>EEVKAIRIPVVRLKFGEVAEATSVVVLPVCKAEEGEKKILEAPMEIIAGGDFKVVEAEKGWKRWVVLPSWNPVAAIGKGGVAVSFRDDRKVLPWDGKEEPLLVVADRVRNVVEADDGYYLVVAENGLKLEKGSDLKAREVKESLGMVVLVVRPPREDDDDWQTSHQ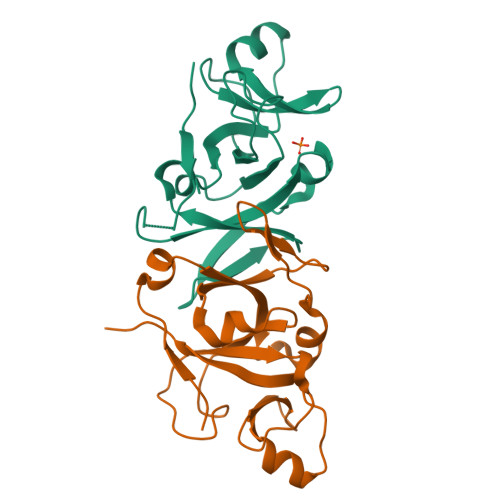NWD[4x]>[2x]MYRTHYSSEITEELNGQKVKVAGWVWEVKDLGGIKFLWIRDRDGIVQITAPKKKVDPELFKLIPKLRSEDVVAVEGVVNFTPKAKLGFEILPEKIVVLNRAETPLPLDPTGKVKAELDTRLNNRFMDLRRPEVMAIFKIRSSVFKAVRDFFHENGFIEIHTPKIIATATEGGTELFPMKYFEEDAFLAESPQLYKEIMMASGLDRVYEIAPIFRAEEHNTTRHLNEAWSIDSEMAFIEDE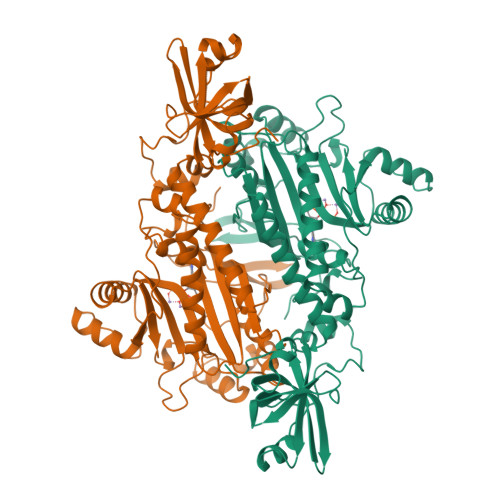EEVMSFLERLVAHAINYVREHNAKELDILNFELEEPKLPFPRVSYDKALEILGDLGKEIPWGEDIDTEGERLLGKYMMENENAPLYFLYQYPSEAKPFYIMKYDNKPEICRAFDLEYRGVEISSGGQREHRHDILVEQIKEKGLNPESFEFYLKAFRYGMPPHGGFGLGAERLIKQMLDLPNIREVILFPRDRRRLTP> AGTAKGHNPTEFPTIYDASSAPTAANTTVGIITIGGVSQTLQDLQQFTSANGLASVNTQTIQTGSSNGDYSDDQQGQGEWDLDSQSIVGSAGGAVQQLLFYMADQSASGNTGLTQAFNQAVSDNVAKVINVSLGWCEADANADGTLQAEDRIFATAAAQGQTFSVSSGDEGVYECNNRGYPDGSTYSVSWPASSPNVIAVGGTTLYTTSAGAYSNETVWNEGLDSNGKLWATGGGYSVYESKPSWQSVVSGTPGRRLLPDISFDAAQGTGALIYNYGQLQQIG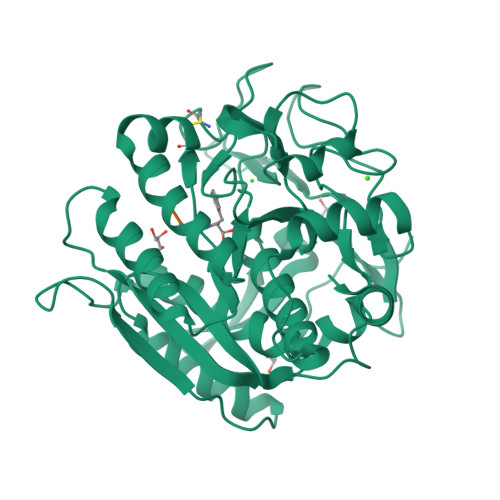GTSLASPIFVGLWARLQSANSNSLGFPAASFYSAISSTPSLVHDVKSGNNGYGGYGYNAGTGWDYPTGWGSLDIAKLSAYIRSNGF>[5x]MGIKDSKINIYYGKNYPFLCRTVFNIYQNNIKKKTANNLNDKKIKEI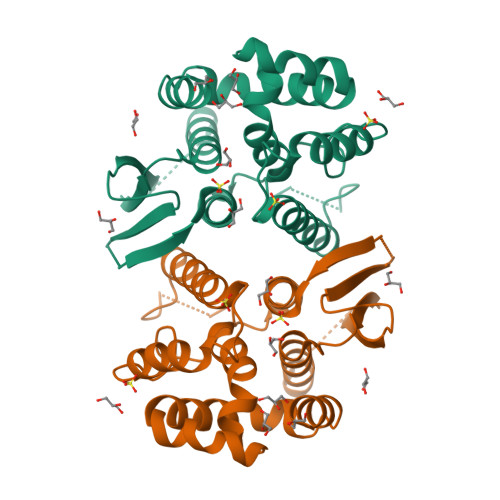CVNFINDKTVVEDIKVEFVRNTVSDQTRKNTNTNNSVTSSDKIFAINLDFLLKTNLYYFTSYRENINRNIITNVFFQAQYNEWIDFLRNKDIEKNIIPICEHINKHLYLNTFLSFHYLTLSDIYIYYEMHKYFSGNITTNLKYPKQYKNINRWFRLIKALLHDHVATDAELIQNLKVKEKIFIDGGSSGLVPRGSSHHHHHH>MGSSHHHHHHSSGLVPRGSHMAASDEARAVSDPAAGWFWQAVARQDLKSVSDALDLDADAPLSATLPALSVWHRQERERVLADGWRYRVDWVRVAPQPVRRTRETWLLVVPPGGIEEALVERLTDALNTRGISTLRLDVPPAATSGELATELRAAADGDPVKAILSLTALDERPHPECKDVPSGIALLLNLVKALGEADLRIPLWTITRGAVKAGPADRLLRPMQAQAWGLGRVAALEHPERWGGLIDLPDSLDGDVLTRLGEALTNGLAEDQLAIRQSGVLARRLVPAPANQPAGRKWRPRGSALITGGLGAVGAQVARWLAEIGAERIVLTSRRGNQAAGAAELEAELRALGAQVSIVACDVTDRAEMSALLAEFDVTAVFHAAGVGRLLPLAETDQNGLAEICAAKVRGAQVLDELCDSTDLDAFVLFSSGAGVWGGGGQGAYGAANAFLDTLAEQRRARGLPATSISWGSWAGGGMADGAAGEHLRRRGIRPMPAASAILALQEVLDQDETCV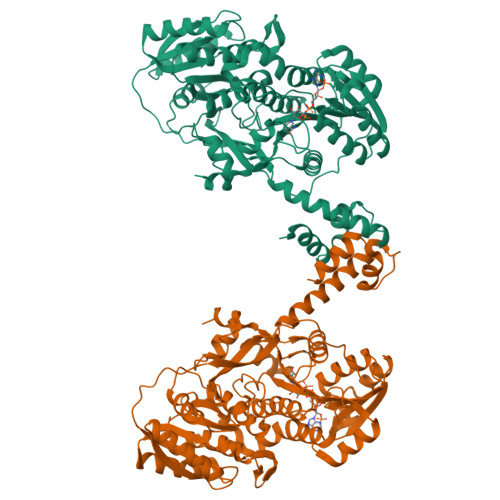SIADVDWDRFVPTFAATRATRLFDEVPAARKAMPANGPAEPGGSPFARNLAELPEAQRRHELV[4x]>MNLKDKILGVAKELFIKNGYNATTTGEIVKLSESSKGNLYYHFKTKENLFLEILNIEQSKWQEQWKKEQIKAKTNREKFYLYNELSLTTEYYYPLQNAIIEFYTEYYKTNSINEKMNKLENKYIDAYHVIFKEGNLNGEWSINDVNAVSKIAANAVN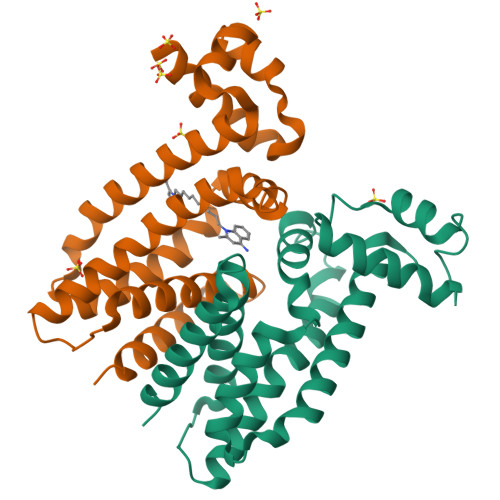GIVTFTHEQNINERIKLMNKFSQIFLNGLSK[4x]2-(2,4-DICHLOROPHENOXY)-5-(3-PHENYLPROPYL)PHENOL 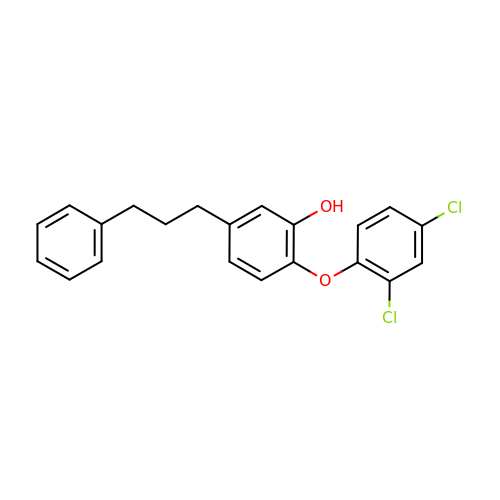| C21 H18 Cl2 O2 | MJRPBNSOVIMDHN-UHFFFAOYSA-N>[2x]ADVSAAVGATGQSGMTYRLGLSWDWDKSWWQTSTGRLTGYWDAGYTYWEGGDEGAGKHSLSFAPVFVYEFAGDSIKPFIEAGIGVAAFSGT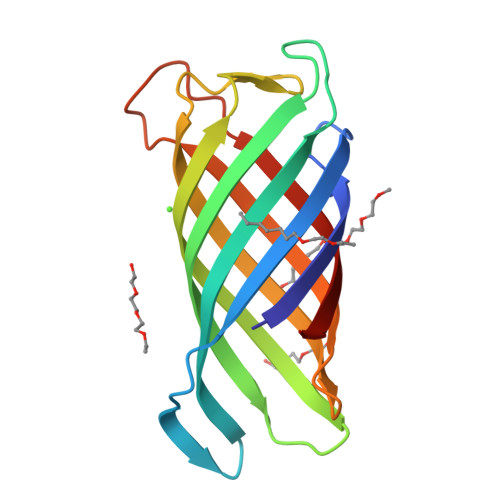RVGDQNLGSSLNFEDRIGAGLKFANGQSVGVRAIHYSNAGLKQPNDGIESYSLFYKIPI6-O-phosphono-alpha-D-allopyranose | C6 H13 O9 P | 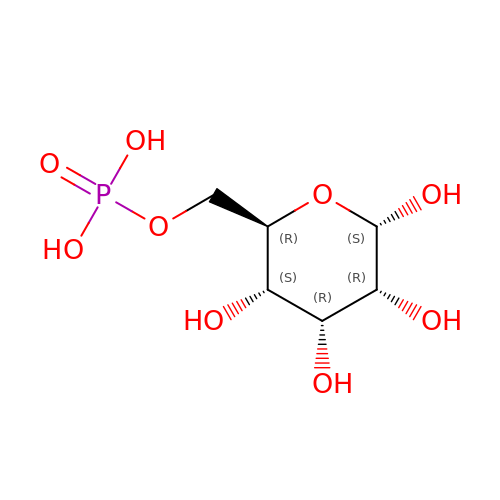NBSCHQHZLSJFNQ-UKFBFLRUSA-N>[6x]MTAPIPVVPVSRPQAKTSLKLPNNQVWVTRKASEWSAKTIDTNDAIPFKTIVEGIPEINSETKFYRLLIGFVAVSDGTFGMVDGVTGDVIPDPPVVGRLGFKKNTYRSRDF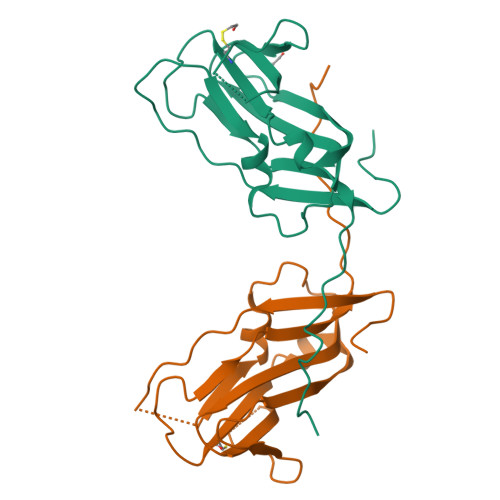DLGGKLLNQLDDRAIVWCLDERRRDAKRVQLAGYWIAISKPAPLMPPEDFLVNQD>[4x]MARLDKSKVINSALELLNEVGIEGLT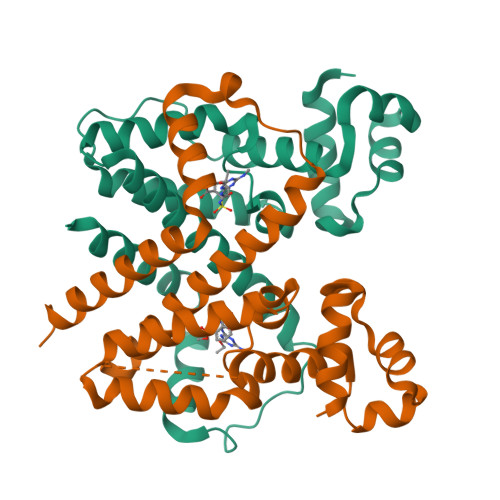TRKLAQKLGVEQPTLYWHVKNKRALLDAMAIEMLDRHATHYSPLERESWQNFLRNNAKSMRNALLSHRDGAKVCLGTGFTEQQYETAENSLAFLTQQGFSLENALYAMQAVGIYTLGCVLLDQELQVAKEERETPTTDSMPPLVRQAVELKDHQGAEPAFLFGLELIIAGLEKQLKCESGS> MAWPKVQPEVNIGVVGHVDHGKTTLVQAITGIWTSKHSEELKRGMT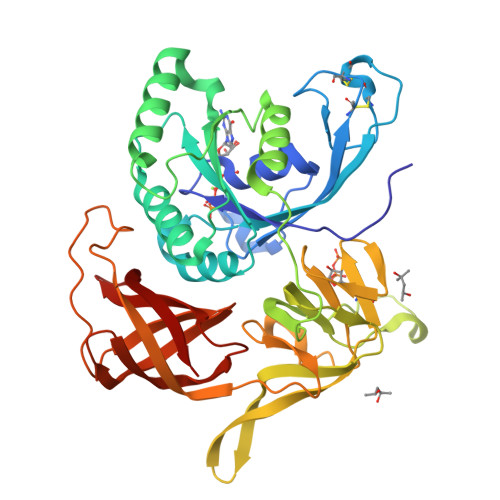IKLGYAETNIGVCESCKKPEAYVTEPSCKSCGSDDEPKFLRRISFIDAPGAEVLMATMLSGAALMDGAILVVAANEPFPQPQTREHFVALGIIGVKNLIIVQNKVDVVSKEEALSQYRQIKQFTKGTWAENVPIIPVSALHKINIDSLIEGIEEYIKTPYRDLSQKPVMLVIRSFDVNKPGTQFNELKGGVIGGSIIQGLFKVDQEIKVLPGLRVEKQGKVSYEPIFTKISSIRFGDEEFKEAKPGGLVAIGTYLDPSLTKADNLLGSIITLADAEVPVLWNIRIKYNLLERVVGAKEMLKVDPIRAKETLMLSVGSSTTLGIVTSVKKDEIEVELRRPVAVWSNNIRTVISRQIAGRWRMIGWGLVEI>[2x]GHMNLCYIDGKFLPLEEAKLPVTDLIIQRGVGVFETISTHSRRPLMLTPHLKRLEGSATASSIVMPATLDEMARIIREGIKKMGCETMVRPYITGGDSFGKDHLFSSSRYFVIFEEIRKPDPILYEKGVALHPINAERYLPSTKSINYMLSFTGQRDSKGAYEILYCPEGEIVEGSHSTFFLIKNGHLITAPTSRALSGTTRQIVLELARRG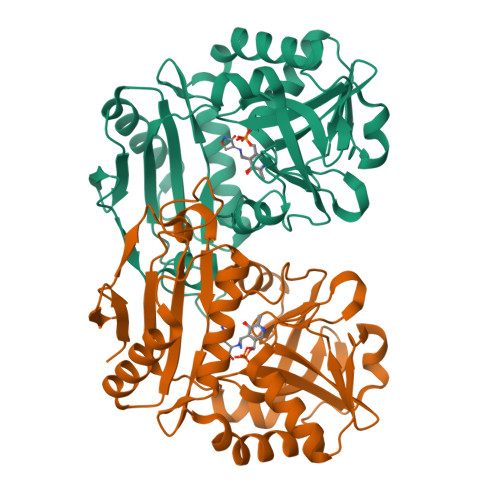NIQVEERCPLLTELPEAEEAFITGTVKELLPVVRIGDQIIGNGVPGKLTKHLHQVYLSSIVEWLE>[4x]RDSCQLVLVESIPQDLPSAAGSPSAQPLGQAWLQLLDTAQESVHVASYYWSLTGPDIGVNDSSSQLGEALLQKLQQLLGRNISLAVATSSPTLARTSTDLQVLAARGAHVRQVPMGRLTRGVLHSKFWVVDGRHIYMGSANMDWRSLTQVKELGAVIYNCSHLAQDLEKTFQTYWVLGVPKAVLPKTWPQNFSSHFNRFQPFHGLFDGVPTTAYFSASPPALCPQGRTRDL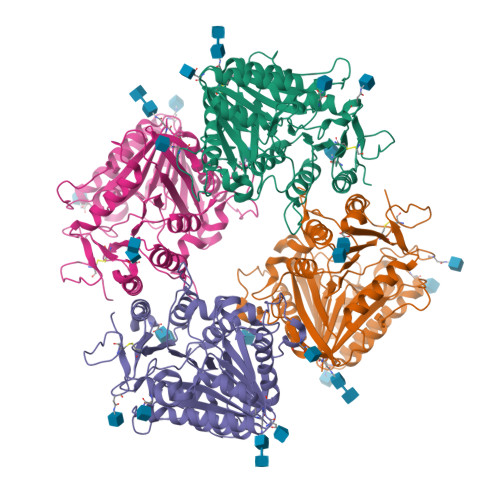EALLAVMGSAQEFIYASVMEYFPTTRFSHPPRYWPVLDNALRAAAFGKGVRVRLLVGCGLNTDPTMFPYLRSLQALSNPAANVSVDVKVFIVPVGNHSNIPFSRVNHSKFMVTEKAAYIGTSNWSEDYFSSTAGVGLVVTQSPGAQPAGATVQEQLRQLFERDWSSRYAVGLDGQAPGQDCVWQGLEVLFQ>[4x]MANIEGVCDQRFSGLKEALARNLDSGEDVGAAIALTIDGESVVDMWGGWVDVEHTAPWSRDTVTNVWSCSKTVTALAALMLVDRGLLDLDAPVAQYWPEFAAAGKDRIRVRQLLSHTSGVSGWDQPFTLENICDDEYATARLATQAPWWEPGTASGYHALNYGHLIGEV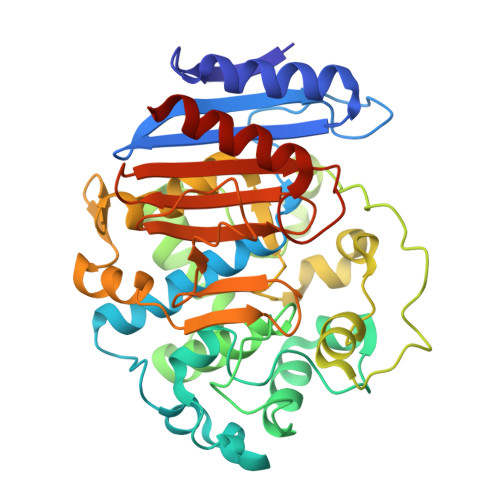VRRIDGRTLGRFIDEEIAGPLDADFRLGLPKSEYGRVSNVIAPPPLPIDIAALGMDNIMVKTFTAPPADATGSWTDGWRAAEIGAANGHSNARALARIQSVIACGGKVGDVRLLSEETIDKIFEEQSYGVDLVLGVPVRFGVGFGLPTPESVPFIPEGRICFWGGWGGSQIIIDTEKRMTFSYVMNKMGPGLLGSERSAQYVSAAYDALSLEHHHHHH>GPSGMILKRAYDVTPQKISTDKVRGVRKRVLIGLKDAPNFVMRLFTVEPGGLIDRASHPWEHEIFVLKGKLTVLKEQGEETVEEG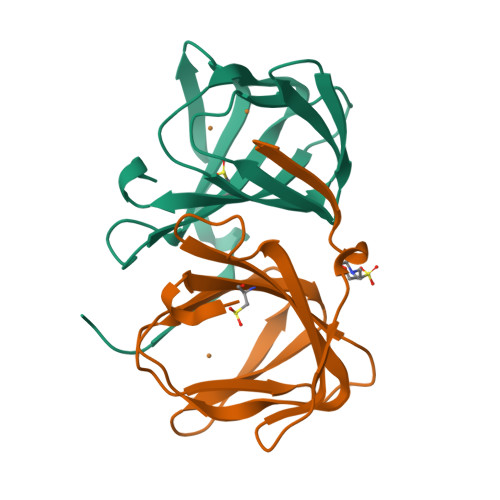FYIFVEPNEIHGFRNDTDSEVEFLCLIPKEGGE[2x]> MGFLELDTNLPANRVPAGLEKRLCAAAASILGKPADRVNVTVRPGLAMALSGSTEPCAQLSISSIGVVGTAEDNRSHSAHFFEFLTKELALGQDRILIRFFPLESWQIGKIGTVMTFL

pmcThe human macrophage migration inhibitory factor (MIF) superfamily, comprised of MIF and D-dopachrome tautomerase (DDT, also called MIF-2), is broadly and constitutively expressed with involvement in proinflammatory and host antimicrobial responses. MIF and MIF-2 are highly similar in structure, with monomeric units of 114 and 117 amino acids, respectively, that form homotrimers. An evolutionarily conserved proline at the N terminus acts as the catalytic base for a tautomerization reaction of unknown biological significance in both proteins. The same site in MIF-2 is Phe100 and is also evolutionarily conserved among all MIF-2 proteins, suggesting this site plays an important role in both proteins.

Mutation of Pro1 abolished activity, supporting the critical role of the N-terminal proline in the HPP enol-keto tautomerase reaction for MIF-2. The P1G MIF-2 variant has no catalytic activity because of the dynamics of the glycine and the altered pKa preventing it from functioning as a catalytic base, which is also observed for P1G MIF. This conclusion is supported by the F100A and S62A variants, which should have the same proline pKa as wt-MIF-2 and possess catalytic activity. We were surprised to find the initiating Met of the P1G MIF-2 variant, as it is cleaved by Escherichia coli methionine aminopeptidase in the P1G MIF protein. Our goal with the P1G variant was to abolish activity and probe the catalytic site's effect on Phe100, and the unexcepted variant with the initiating Met still serves that role. Crystal structures of MIF variants and substrate- or inhibitor-bound complexes typically display very few differences, and consistent with this trend, the P1G and S62A variants have RMSD values of 0.30 Å and 0.32 Å with the wt-MIF-2 trimer, respectively. P1G also has an extensive water network, but whatever effect this might have on catalytic activity is abolished by the removal of Pro1. Proline 1 mutation has a large influence on the MIF-2 structure in solution, whereas the F100A mutant had more modest chemical shift perturbations by comparison. The P1G variant logically perturbed Phe2; however, it also caused broadening at Ser62 and chemical shift perturbations at Phe100 and selected sites near flexible loops and the C-terminus. However, subtle elevation in the dynamics of residues 20 to 30 distal to the monomer–monomer interface and decreases in residues 60 to 75 surrounding the allosteric pathway along the solvent cavity are observed in P1G MIF-2.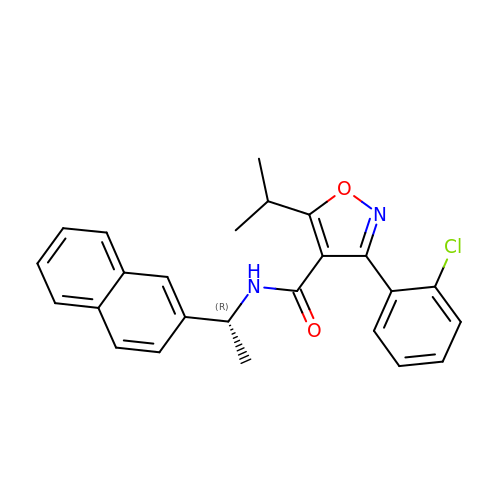3-(2-chlorophenyl)-N-[(1R)-1-(naphthalen-2-yl)ethyl]-5-(propan-2-yl)-1,2-oxazole-4-carboxamide | C25 H23 Cl N2 O2 | OKVWUQCQUFGLKM-MRXNPFEDSA-N>WEETKECAFTEFFKLAPLASNPALSVCQDASGWQMLPPAGYPTPEQLKLMCGTAECFTLIDAIK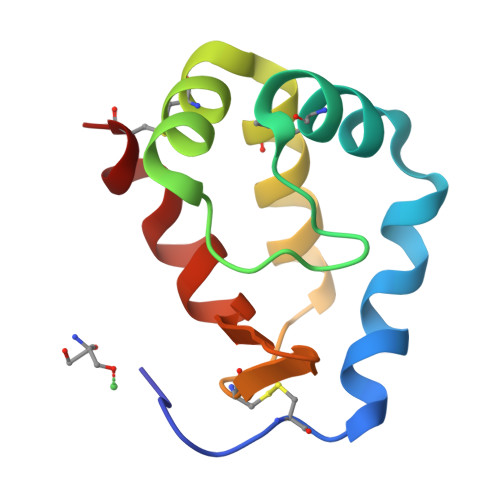ALNPNDCILVFGDVRLNVKKLVTEFEPSCF[2x]> SSQIRQNYSTEVEAAVNRLVNLYLRASYTYLSLGFYFDRDDVALEGVCHFFRELAEEKREGAERLLKMQNQRGG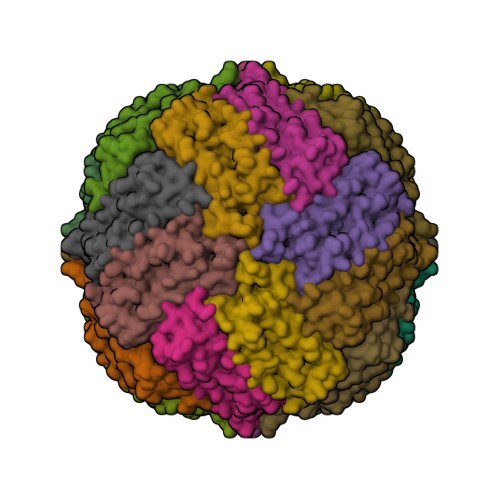RALFQDLQKPSQDEWGTTLDAMKAAIVLEKSLNQALLDLHALGSAQADPHLCDFLESHFLDEEVKLIKKMGDHLTNIQRLVGSQAGLGEYLFERLTLKHD>MLNPIVRKFQYGQHTVTLETGMMARQATAAVMVSMDDTAVFVTVVGQKKAKPGQDFFPLTVNYQERTYAAGRIPGSFFRREGRPSEGETLIARLIDRPIRPLFPEGFVNEVQVIATVVSVNPQVNPDIVAMIGASAALSLSGIPFNGPIGAARVGYINDQYVLNPTQDELKESKLDLVVAGTEAAVLMVESEAQLLSEDQMLGAVVFGHEQQQVVIQNINELVKEAGKPRWDWQPEPVNEALNARVAALAEARLSDAYRITDKQERYAQVDVIKSETIATLLAEDETLDENELGEILHAIEKNVVRSRVLAGEPRIDGREKDMIRGLDVRTGVLPRTHGSALFTRGETQALVTATLGTARDAQVLDELMGERTDTFLFHYNFPPYSVGETGMVGSPKRREIGHGRLAKRGVLAVMPDMDKFPYTVRVVSEITESNGSSSMASVCGASLALMDAGVPIKAAVAGIAMGLVKEGDNYVVLSDILGDEDHLGDMDFKVAGSRDGISALQMDIKIEGITKEIMQVALNQAKGARLHILGVMEQAINAPRGDISEFAPRIHTIKINPDKIKDVIGKGGSVIRALTEETGTTIEIEDDGTVKIAATDGEKAKHAIRRIEEITAEIEVGRVYTGKVTRIVDFGAFVAIGGGKEGLVHISQIADKRVEKVTDYLQMGQEVPVKVLEVDRQGRIRLSIKEATEQSQPAAAPEAPAAEQGE[3x]

Polynucleotide phosphorylase (PNPase) is an ancient exoribonuclease conserved in the course of evolution and is found in species as diverse as bacteria and humans. Although PNPase can catalyze the polymerization of nucleotides, its main cellular function is the 3ʹ-to-5ʹ degradation of RNA (Grunberg-Manago et al., 1955). While the catalytic core performs the phosphorolytic action, the KH and S1 domains participate in RNA substrate capture and autoregulation (Wong et al., 2013) and are powerful facilitators of PNPase activity. Cryoelectron microscopy (cryo-EM) was used to solve structures for E. coli PNPase in the apo- and substrate-bound forms and in a ternary complex with sRNA substrate and Hfq (i.e., the RNA carrier complex).

Cryo-EM studies were carried out on complexes formed between PNPase and RNA under conditions that do not support catalysis. We used the sponge RNA 3ʹETSleuZ, which was observed in vivo in pull-downs of PNPase under conditions of induced RyhB expression. Comparison of the models for PNPase-RNA and apo-PNPase shows that both KH and S1 domains clamp onto the 3ʹETSleuZ substrate. In particular, one of the three KH domains appears to be the main contact for the RNA substrate. Although density for RNA is not apparent within the active sites of the enzyme, there is visible density for three bases stacking on the three Phe77 residues at the entrance channel, where the RNA path may branch among three possible routes into the core interior (Figure 1Diii). The structure of the substrate-bound enzyme in the phosphorolytic mode indicates how the flexibility of the S1 and KH domains facilitates substrate capture and how these domains clamp down on intercepted single-stranded RNA.> SSYSGPIVVDPVTRIEGHLRIEVEVENGKVKNAYSSSTLFRGLEIILKGRDPRDAQHFTQRTCGVCTYTHALASTRCVDNAVGVHIPKNATYIRNLVLGAQYLHDHIVHFYHLHALDFVDVTAALKADPAKAAKVASSISPRKTTAADLKAVQDKLKTFVETGQLGPFTNAYFLGGHPAYYLDPETNLIATAHYLEALRLQVKAARAMAVFGAKNPHTQFTVVGGVTCYDALTPQRIAEFEALWKETKAFVDEVYIPDLLVVAAAYKDWTQYGGTDNFITFGEFPKDEYDLNSRFFKPGVVFKRDFKNIKPFDKMQIEEHVRHSWYEGAEARHPWKGQTQPKYTDLHGDDRYSWMKAPRYMGEPMETGPLAQVLIAYSQGHPKVKAVTDAVLAKLGVGPEALFSTLGRTAARGIETAVIAEYVGVMLQEYKDNIAKGDNVICAPWEMPKQAEGVGFVNAPRGGLSHWIRIEDGKIGNFQLVVPSTWTLGPRCDKNKLSPVEASLIGTPVADAKRPVEILRTVHSFDPCIACGVH;> LMGPRRPSVVYLHNAECTGCSESVLRAFEPYIDTLILDTLSLDYHETIMAAAGDAAEAALEQAVNSPHGFIAVVEGGIPTAANGIYGKVANHTMLDICSRILPKAQAVIAYGTCATFGGVQAAKPNPTGAKGVNDALKHLGVKAINIAGCPPNPYNLVGTIVYYLKNKAAPELDSLNRPTMFFGQTVHEQCPRLPHFDAGEFAPSFESEEARKGWCLYELGCKGPVTMNNCPKIKFNQTNWPVDAGHPCIGCSEPDFWDAMTPFY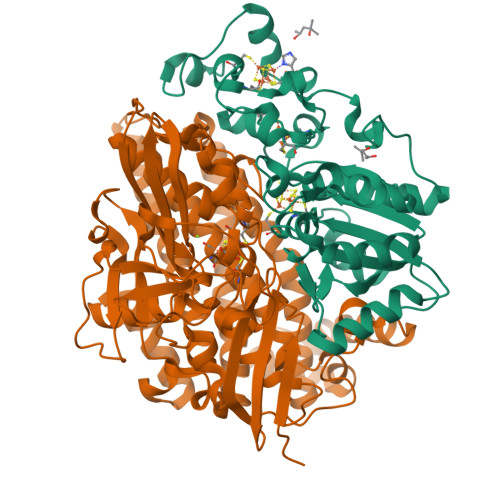QN>MNHKVHMMSQPKPILYYDERSPPVRSCLMLIKLLDIDVELRFVNLFKGEQFQKDFLALNPQHSVPTLVHGDLVLTDSHAILIHLAEKFDEGGSLWPQEHAERMKVLNLLLFECSFLFRRDSDFMSAIVRQGFANVDVAHHERKLTEAYIIMERYLENSDFMAGPQLTLADLSIVTTLSTV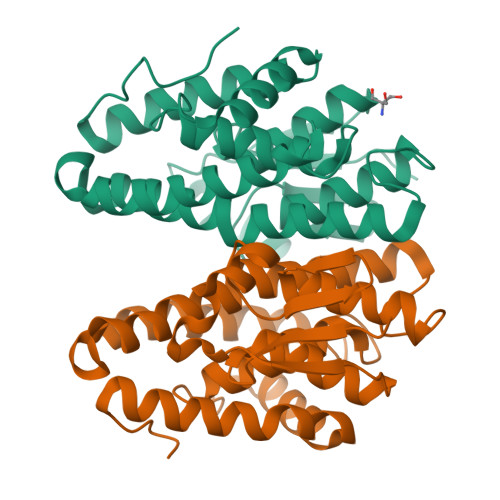NLMFPLSQFPRLRRWFTAMQQLDAYEANCSGLEKLRQTMESVGSFQFPSSSAVVTEKVE[2x]> GKKSRMCGYCGAPAPYATACGLDVCVYHTHFHQHCPVIIWCGHPAGSGSCSECEPPLGKGTSPLDEVLEQVPYKPPRTVIMHVEQGLTPLDPGRYQTRRGLVSVRRGIRGNEVDLPDGDYASTALLPTCKEINMVAVASNVLRSRFIIGPPGAGKTHWLLQQVQDGDVIYTPTHQTMLDMIRALGTCRFNVPAGTTLQFPAPSRTGPWVRILAGGWCPGKNSFLDEAAYCNHLDVLRLLSKTTLTCLGDFKQLHPVGFDSHCYVFDIMPQTQLKTIWRFGQNICDAIQPDYRDKLMSMVNTTRVTYVEKPVRYGQVLTPYHRDREDSAITIDSSQGATFDVVTLHLPTKDSLNRQRALVAITRARHAIFVYDPHRQLQSVFDLPAKGTPVNLAVHRDEQLIVLDRNNREITVAQALGNGDKFRATDKRVVDSLRAICADLE

Nsp10 belongs to the superfamily 1B (SF1B) Upf1-like family of helicases, which could unwind both DNA and RNA duplexes. In addition, this family of helicases contains an N-terminal predicted zinc-binding domain (ZBD) which is conserved in all nidovirus helicases, including 12 or 13 conserved Cys and His residues. In this paper, we present the structure of HP-PRRSV nsp10 in full length and truncation, which has a different domain arrangement compared with other helicases. The N-terminal ZBD has 13 conserved Cys/His residues, twelve of which participate in the coordination of three zinc ions.

The diffraction of the crystals of full-length HP-PRRSV nsp10 was poor after extensive optimization. However, after conducting the lysine methylation protocol, the resolution was greatly improved from 10 to 2.5 Å. Basic Local Alignment Search Tool (BLAST) searches of the PRRSV nsp10 sequence among the solved structures in the PDB database revealed that the sequence identities with known structures were low, with the highest value being only 30%. Moreover, the structure could not be solved using the closest homologs as search models after extensive trials by molecular replacement. We determined the structure by single-wavelength anomalous dispersion (SAD) phasing using the signals from the Zn atoms. Comparison of these three structures showed that all the overall domain arrangement was similar, except that the truncated form lacked the C-terminal 168 residues due to the degradation during the period of crystallization.> MVDAFTTSKVTLSTTGNAQEPAGRFTKVAAAVADSVVTIESVSDQEGMQGSGVIVDGRGYIVTNNHVISEAANNPSQFKTTVVFNDGKEVPANLVGRDPKTDLAVLKVDNVDNLTVARLGDSSKVRVGDEVLAVGAPLGLRSTVTQGIVSALHRPVPLSGEGSDTDTVIDAIQTDASINHGNAGGPLIDMDAQVIGINTAGKSLSDSASGLGFAIPVNEMKLVANSLIKDGKIVHPTLGISTRSVSNAIASGAQVANVKAGSPAQKGGILENDVIVKVGNRAVADSDEFVVAVRQLAIGQDAPIEVVREGRHVTLTVKPDPDSTKLAAALEHHHH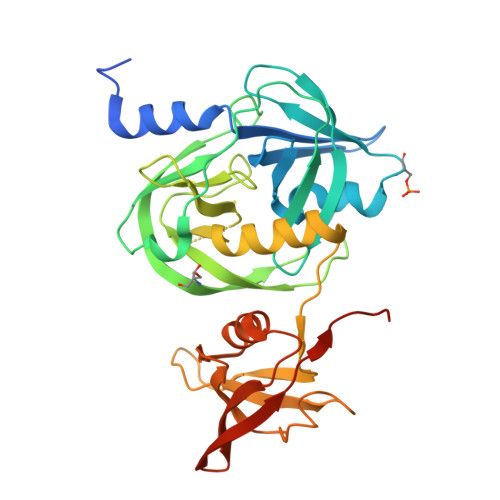HH> MKAKVIDAVSFSYILRTVGDFLSEANFIVTKEGIRVSGIDPSRVVFLDIFLPSSYFEG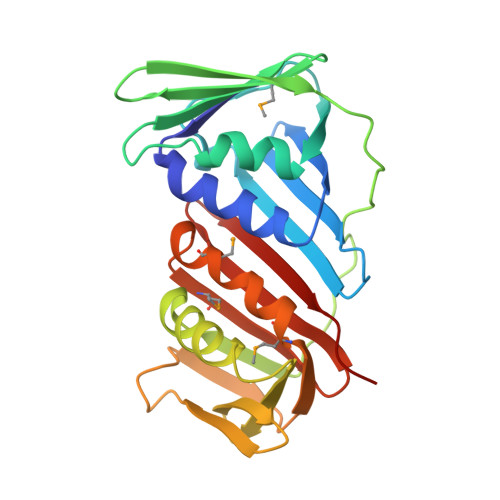FEVSQEKEIIGFKLEDVNDILKRVLKDDTLILSSNESKLTLTFDGEFTRSFELPLIQVESTQPPSVNLEFPFKAQLLTITFADIIDELSDLGEVLNIHSKENKLYFEVIGDLSTAKVELSTDNGTLLEASGADVSSSYGMEYVANTTKMRRASDSMELYFGSQIPLKLRFKLPQEGYGDFYIAPRAD> GFPTEPKPGTNQFLTTDDGVSAPILPNFHPTPCIHIPGEVRNLLELCQVETILEVNNVPTNATSLMERLRFPVSAQAGKGELCAVFRADPGRDGPWQSTMLGQLCGYYTQWSGSLEVTFMFTGSFMATGKMLIAYTPPGGPLPKDRATAMLGTHVIWDFGLQSSVTLVIPWISNTHYRAHARDGVFDYYTTGLVSIWYQTNY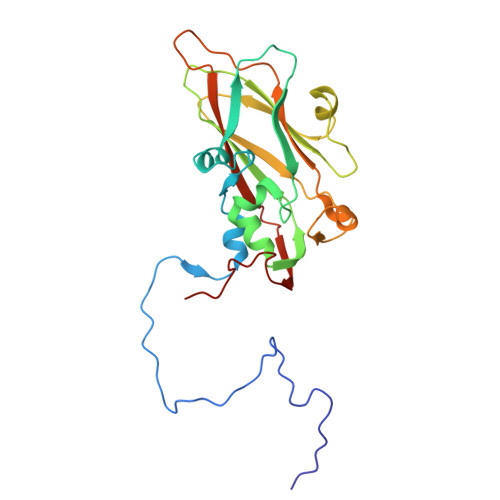VVPIGAPNTAYIIALAAAQKNFTMKLCKDTSHILQTASIQ>[2x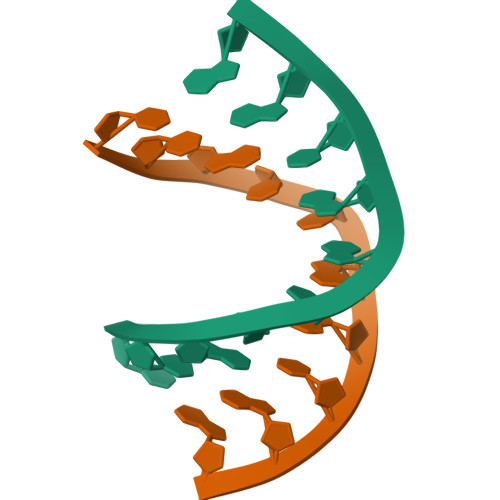]CCACTAGTGG>[2x]MNPDREGWLLKLGGRVKTWKRRWFILTDNCLYYFEYTTDKEPRGIIPLENLSIREVEDPRKPNCFELYNPSHKGQVIKACKTEADGRVVEGNHVVYRISAPSPEEKEEWMKSIKASISRD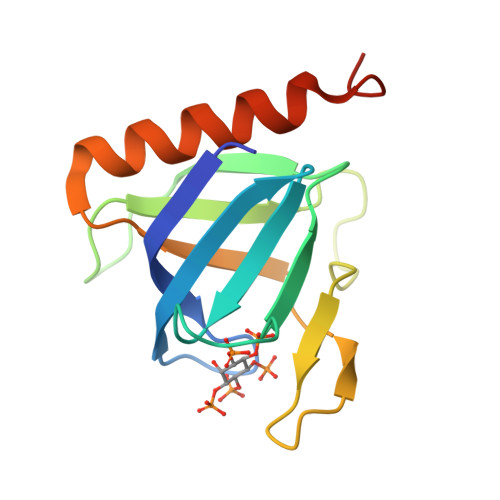PFYDMLATR>AMAGVYTYENEFTSDIPAPKLFKAFVLDADNLIPKIAPQAVKCAEILEGDGGPGTIKKITFGEGSHYGYVKHKIHSIDKVNHTYSYSLIEGDALSENIEKIDYETKLVSAPHGGTIIKTTSKYHTKGDVEIKEEHVKAGKEKAAHLFKLIEGYLKDHP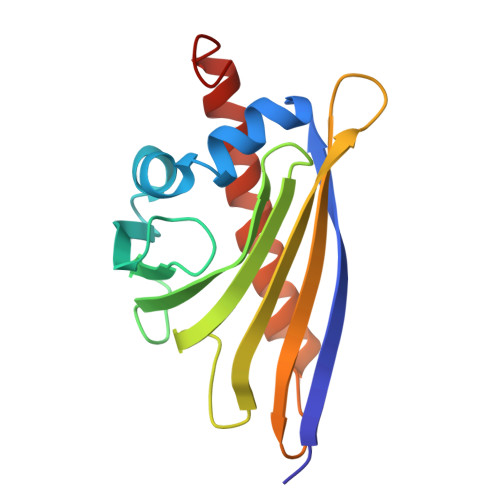SEYN[6x]> LTEIEHLVQSVCKSYRETCQLRLEDLLRQRSNIFSREEVTGYQRKSMWEMWERCAHHLTEAIQYVVEFAKRLSGFMELCQNDQIVLLKAGAMEVVLVRMCRAYNADNRTVFFEGKYGGMELFRALGCSELISSIFDFSHSLSALHFSEDEIALYTALVLINAHRPGLQEKRKVEQLQYNLELAFHHHLHKTHRQS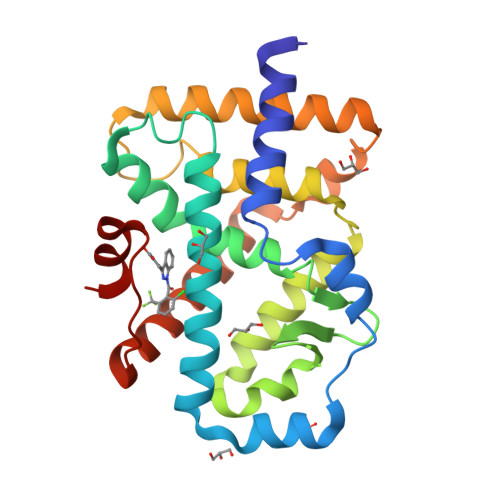ILAKLPPKGKLRSLCSQHVERLQIFQHLHPIVVQAAFPPLYKELFS> GPSLKSPLKPESQLDLRVQELIKLICNVQAMEEMMMEMKYNTKKAPLGKLTVAQIKAGYQSLKKIEDCIRAGQHGRALMEACNEFYTRIPHDFGLRTPPLIRTQKELSEKIQLLEALGDIEIAIKLVKTELQSPEHPLDQHYRNLHCALRPLDHESYEFKVISQYLQSTHAPTHSDYTMTLLDLFEVEKDGEKEAFREDLHN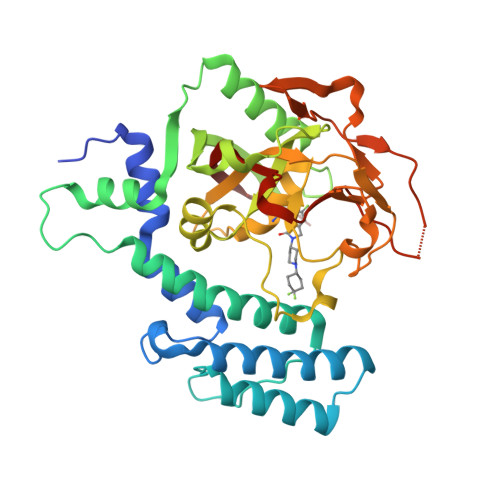RMLLWHGSRMSNWVGILSHGLRIAPPEAPITGYMFGKGIYFADMSSKSANYCFASRLKNTGLLLLSEVALGQCNELLEANPKAEGLLQGKHSTKGLGKMAPSSAHFVTLNGSTVPLGPASDTGILNPDGYTLNYNEYIVYNPNQVRMRYLLKVQFNFLQLW> ANSLVEEFKSGNIERECIEERCSKEEAREVFEDDEKTETFWNVYVDGDQCSSNPCHYRGICKDGIGSYTCTCLSGYEGKNCERV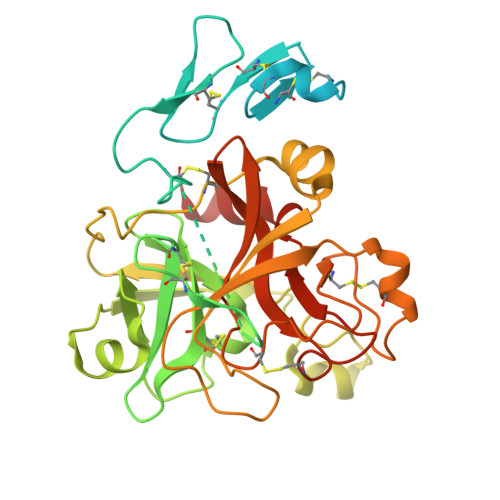LYKSCRVDNGNCWHFCKHVQNDIQCSCAEGYLLGEDGHSCVAGGNFSCGRNIKTRNKREANLPDFVQSQNATLLKKSDNPSPDIRIVNGMDCKLGECPWQAALVDEKEGVFCGGTILSPIYVLTAAHCINETETISVVVGEIDKSRIETGPLLSVDKIYVHKKFVPPQKAYKFDLAAYDYDIAIIQMKTPIQFSENVVPACLPTADFANQVLMKQDFGIVSGFGRIVEKGPKSKTLKVLKVPYVDRHTCMVSSETPITPNMFCAGYDTLPRDACQGDSGGPHTTVYRDTHFITGIVSSGEGCARNGKYGNYTKLSKFIPWIKRIMRQKLPSTESSTGRL N-{2-methoxy-4-[(1-methylpiperidin-4-yl)oxy]phenyl}-4-(1H-pyrrolo[2,3-c]pyridin-3-yl)pyrimidin-2-amine | C24 H26 N6 O2 | 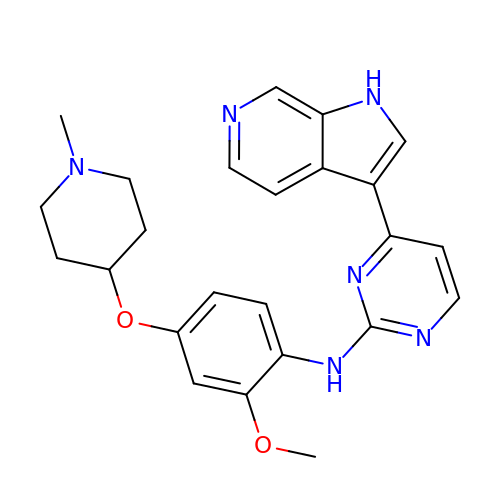FTZQWKAIKYEWPM-UHFFFAOYSA-N> GSMDRKVAREFRHKVDFLIENDAEKDYLYDVLRMYHQTMDVAVLVGDLKLVINEPSRLPLFDAIRPLIPLKHQVEYDQLTPRRSRKLKEVRLDRLHPEGLGLSVRGGLEFGCGLFISHLIKGGQADSVGLQVGDEIVRINGYSISSCTHEEVINLIRTKKTVSIKVRHI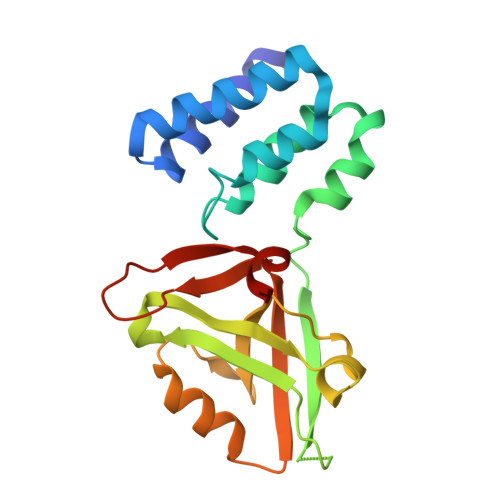GLIPVKSSPDEPLTWQYVDQFVSESGG> MEKIGETMAKLGQNTRVNSDQLIQTILADPEVASFISQHHLSQEQINLSLSKFNQFLVERQKYQLKDPSYIAKGYQPILAMNEGYADVSYLETKELVEAQKQAAISERIQLVSLPKSYRHIHLSDIDVNNASRMEAFSAILDFVEQYPSAEQKGLYL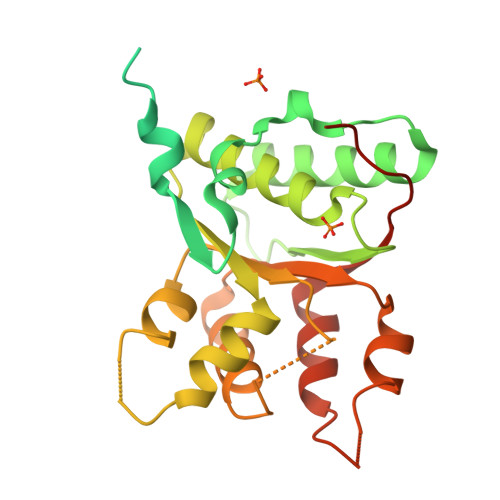YGDMGIGKSYLLAAMAHELSEKKGVSTTLLHFPSFAIDVKNAISNGSVKEEIDAVKNVPVLILDDIGAEQATSWVRDEVLQVILQYRMLEELPTFFTSNYSFADLERKWATIKGSDETWQAKRVMERVRYLAREFHLEGANRRLEHHHHHH>NPCIEVVPNITYQCMDQKLSKVPDDIPSSTKNIDLSFNPLKILKSYSFSNFSELQWLDLSRCEIETIEDKAWHGLHHLSNLILTGNPIQSFSPGSFSGLTSLENLVAVETKLASLESFPIGQLITLKKLNVAHNFIHSCKLPAYFSNLTNLVHVDLSYNYIQTITVNDLQFLRENPQVNLSLDMSLNPIDFIQDQAFQGIKLHELTLRGNFNSSNIMKTCLQNLAGLHVHRLILGEFKDERNLEIFEPSIMEGLCDVTIDEFRLTYTNDFSDDIVKFHCLANVSAMSLAGVSIKYLEDVPKHFKWQSLSIIRCQLKQFPTLDLPFLKSLTLTMNKGSISFKKVALPSLSYLDLSRNALSFSGCCSYSDLGTNSLRHLDLSFNGAIIMSANFMGLEELQHLDFQHSTLKRVTEFSAFLSLEKLLYLDISYTNTKIDFDGIFLGLTSLNTLKMAGNSFKDNTLSNVFANTTNLTFLDLSKCQLEQISWGVFDTLHRLQLLNMSHNNLLFLDSSHYNQLYSLKELALDTNQLKSVPDGIFDRLTSLQKIWLHTNPWDCSCPRIDYLSRWLNKNSQKEQGSAKCSGSGKPVRSIICPT[2x];>[2x]EKQQWFCNSSDAIISYSYCDHLKFPISISSEPCIRLRG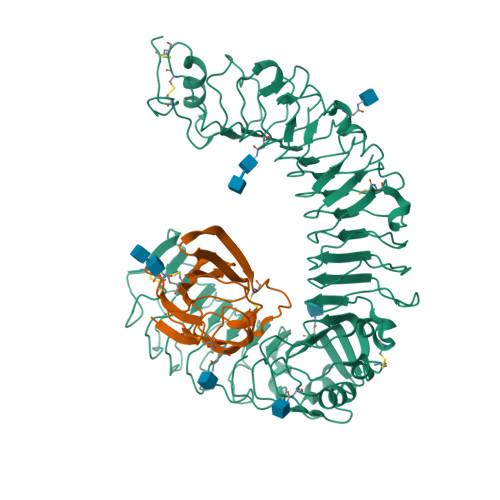TNGFVHVEFIPRGNLKYLYFNLFISVNSIELPKRKEVLCHGHDDDYSFCRALKGETVNTSIPFSFEGILFPKGHYRCVAEAIAGDTEEKLFCLNFTIIHRRDVNKGENLYFQ> SPTINFINFNQTGTCISLGTSKGFKIFNCEPFGKFYSEDSGGYAIVEMLFSTSLLALVGIGDQPALSPRRLRIINTKKHSIICEVTFPTSILSVKMNKSRLVVLLQEQIYIYDINTMRLLHTIETNPNPRGLMAMSPSVANSYLVYPSPPKVINSEIKAHATTNNITLSVGGNTETSFKRDQQDAGHSDISDLDQYSSFTKRDDADPTSSNGGNSSIIKNGDVIVFNLETLQPTMVIEAHKGEIAAMAISFDGTLMATASDKGTIIRVFDIETGDKIYQFRRGTYATRIYSISFSEDSQYLAVTGSSKTVHIFKLGHSMSNNKLDSDDSNMEEAAADDSSLDTTSIDALSDEENPTRLAREPYVDASRKTMGRMIRYSSQKLSRRAARTLGQIFPIKVTSLLESSRHFASLKLPVETNSHVMTISSIGSPIDIDTSEYPELFETGNSASTESYHEPVMKMVPIRVVSSDGYLYNFVMDPERGGDCLILSQYSILM

Autophagy-related protein 18 (Atg18) participates in the elongation of early autophagosomal structures in concert with Atg2 and Atg9 complexes. Atg18 belongs to the protein family of β-propellers that bind polyphosphoinositides (PROPPIN). The corresponding primary structure contains a series of conserved WD40 repeats forming the 6 or 7 blades of a β-propeller fold. The autophagic membrane adapter Atg18 reveals an unexpected structural plasticity in multiple modes of oligomeric organization.

Using these preparations in high-salt buffer, we determined the single-particle cryo-EM structure of soluble Atg18-WT fractions. Due to the very small particle size, i.e., the Atg18 monomer corresponds to 55 kDa, we imaged over 1000 particles on a single cryo-micrograph. Classification analysis revealed separate views of single Atg18 displaying characteristic structural features of blade separation of the β-propeller. Alongside Atg18 monomer particles, we were also able to classify a selection of Atg18 dimers. Comparison with projections of the T and I-interface dimers extracted from atomic model of the Atg18 tube matched some of the 2D classes. Moreover, we failed to reconstruct coherent dimer 3D structures of these Atg18 dimers presumably due to higher flexibility in solution than observed in the helical assembly. Nevertheless, using monomeric class members we determined the 3D structure of Atg18-WT at 4.8 Å resolution according to the FSC 0.143 criterion. Next, we successfully docked a single refined atomic model taken from the helically assembled Atg18 into the density of monomeric Atg18-WT. In accordance with the helical assembly structure, three major loop regions were not resolved and disordered in monomeric Atg18. Together, the structure determination of soluble Atg18 supports the occurrence of monomers and dimers in agreement with the T and I-interfaces observed in the helically assembled lattice structures.> SANEDMPVEKILEAELAVEPKTETYVEANMGLNPSSPNDPVTNICQAADKQLFTLVEWAKRIPHFSELPLDDQVILLRAGWNELLIASASHRSIAVKDGILLATGLHVHRNSAHSAGVGAIFDRVLTELVSKMRDMQMDKTELGCLRAIVLFNPDSKGLSNPAEVEALREKVYASLEAYCKHKYPEQPGRFAKLLLRLPALRSIGLKCLEHLFFFKLIGDTPIDTFLMEMLEA;> PEVGELIEKVRKAHQETFPALCQLGKYTTNNSSEQRVSLDIDLWDKFSELSTKCIIKTVEFAKQLPGFTTLTIADQITLLKAACLDILILRICTRYTPEQDTMTFSDGLTLNRTQMHNAGFGPLTDLVFAFANQLLPLEMDDAETGLLSAICLICGDRQDLEQPDRVDMLQEPLLEALKVYVRKRRPSRPHMFPKMLMKITDLRSISAKGAERVITLKMEIPGSMPPLI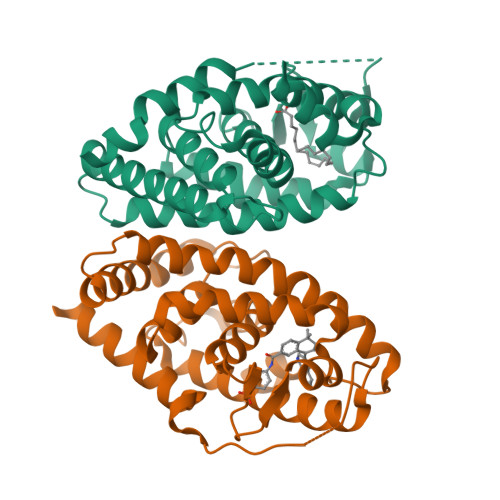QEMLEN N-[(biphenyl-4-yloxy)acetyl]-beta-D-glucopyranosylamine 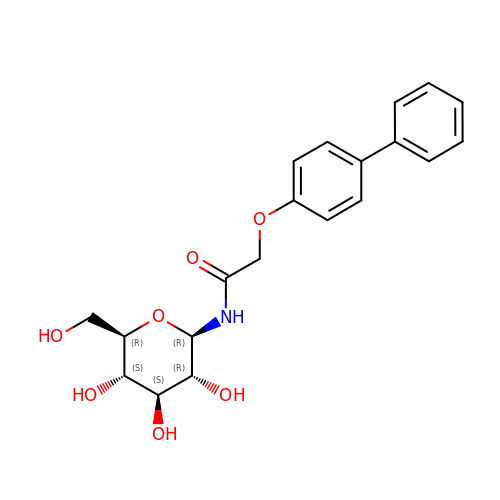| C20 H23 N O7 | NSADEBQKFSASLM-XIKSMUEASA-N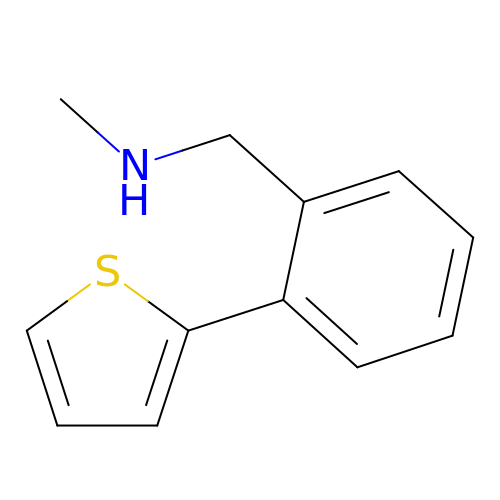N-methyl-1-(2-thiophen-2-ylphenyl)methanamine | C12 H13 N S | MRKJJEJYTBOUTH-UHFFFAOYSA-N>[3x]GVPEGGEETEKAEEDIVMKEKPKVTLNEIVGLEDVKEALKEAVVYPSKRP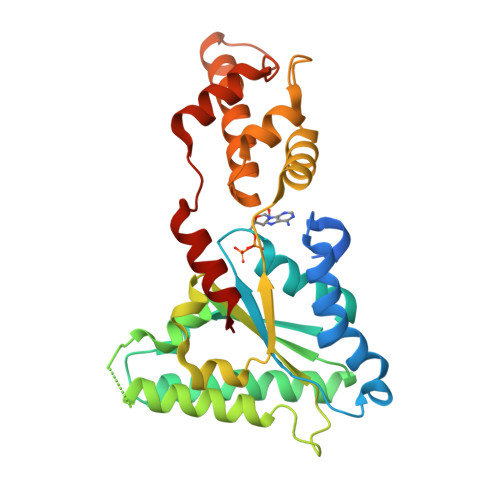DLFPLGWPRGILLYGPPGCGKTMIAAAVANELDSEFIHVDAASIMSKWLGEAEKNVAKIFKTARELSKKENKPAIIFIDELDALLASYTSEVGGEARVRNQFLKEMDGLADKNEISKVYVIGATNKPWRLDEPFLRRFQKRIYITLPDKAHRLELLKHYSSKVKLDPNVNLEELAELTDGYTASDIRDIVQSAHMRVVKEMFEKNLQEPRAINMDDFREVLKVRKPSVNQDMLKAYAAWHEKFKAL> DIYQ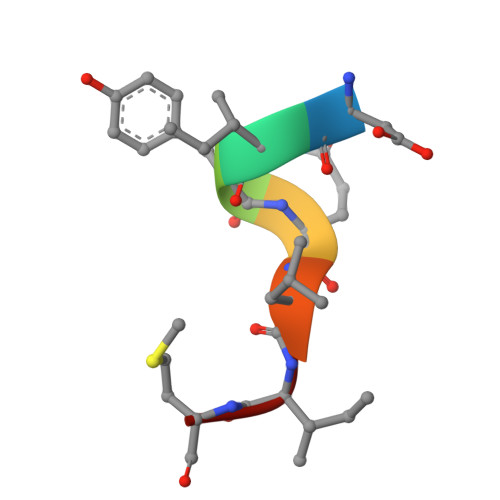LIM>AACLPDIIFDEPSQGPEKNEAISMLTERLSSIINAAGGDIGIAVIHVETGHTTAIQGTTQLPLQSVFKLPLAIAVLKEIEENRLQLDRKVRVTPADVAPGWTANAAMWRRPIDRTVAQLIEVSIIRSDNTSSDKLLQLVGGPAAVTHRMRALGFPNIEIVSTEREFSENRTRPNTGSAEDLARLLVQLQKGELLQPQHSALLLGFMHRATTGTERLRGSLPVGTPVADKTGTGDAGVVTNDVGIITLPKGQGHLAIAVLISGSKLSPAAQEKLIAEIARAAYDAHVSRAE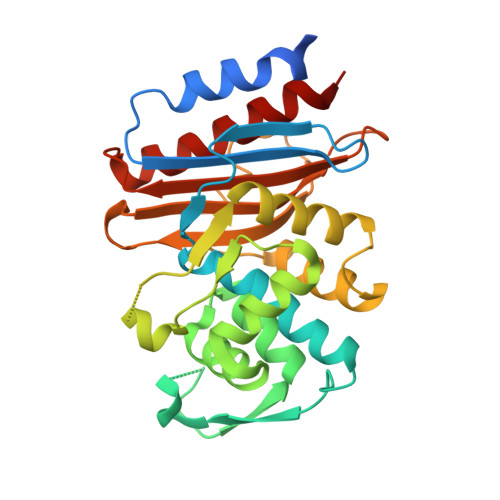[2x]2-((9H-PURIN-6-YLTHIO)METHYL)-5-CHLORO-3-(2-METHOXYPHENYL)QUINAZOLIN-4(3H)-ONE 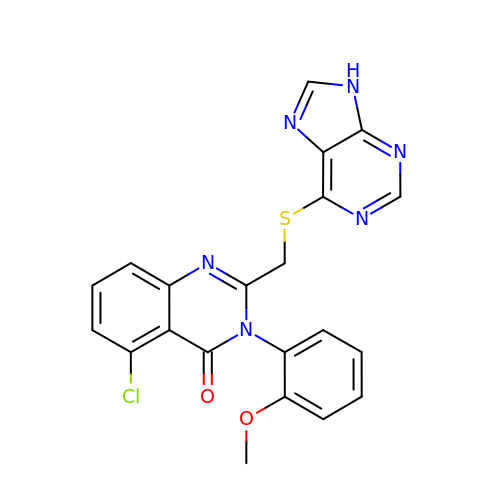| C21 H15 Cl N6 O2 S | UMMYTDJYDSTEMB-UHFFFAOYSA-N> AIEVKDVTDTTALITWSDDFGE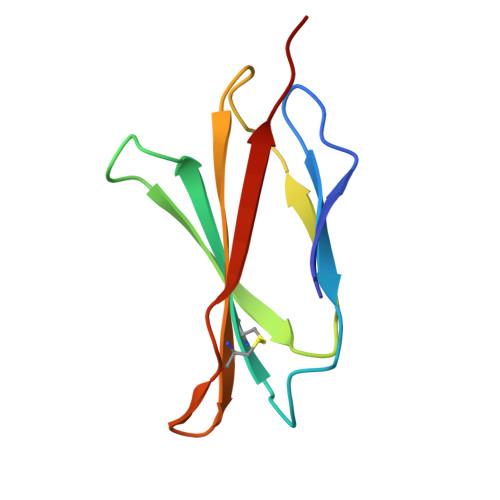YVWCELTYGIKDVPGDRTTIDLWYHHAHYSIGNLKPDTEYEVSLICRRGDMSSNPAKETFTTGLV>MNQSCPNKTSFKIAFIQARWHADIVDEARKSFVAELAAKTGGSVEVEIFDVPGAYEIPLHAKTLARTGRYAAIVGAAFVIDGGIYDHDFVATA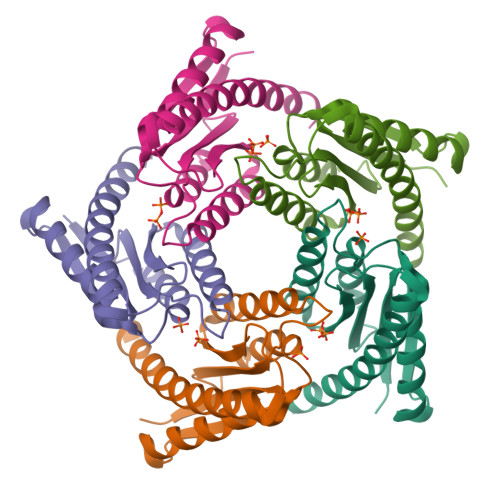VINGMMQVQLETEVPVLSVVLTPHHFHESKEHHDFFHAHFKVKGVEAAHAALQIVSERSRIAALV[5x]> NHAANKSSASRADVKPVTVKLVDSQATMETRSLFAFMQEQRRHSIMFGHQHETTQGLTITRTDGTQSDTFNAVGDFAAVYGWDTLSIVA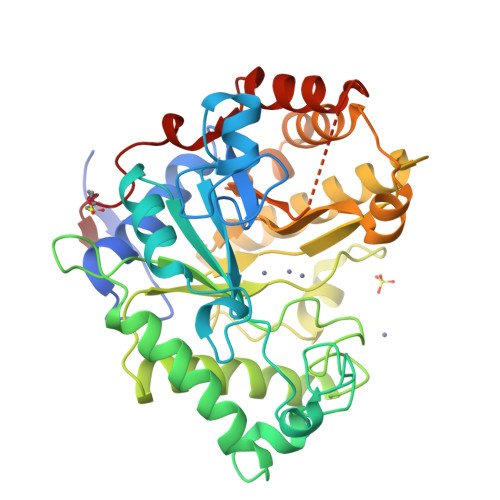PKAEGDIVAQVKKAYARGGIITVSSHFDNPKTDTQKGVWPVGTSWDQTPAVVDSLPGGAYNPVLNGYLDQVAEWANNLKDEQGRLIPVIFRLYHENTGSWFWWGDKQSTPEQYKQLFRYSVEYLRDVKGVRNFLYAYSPNNFWDVTEANYLERYPGDEWVDVLGFDTYGPVADNADWFRNVVANAALVARMAEARGKIPVISEIGIRAPDIEAGLYDNQWYRKLISGLKADPDAREIAFLLVWRNAPQGVPGPNGTQVPHYWVPANRPENINNGTLEDFQAFYADEFTAFNRDIEQVYQRPTLIVK>MPNKITKEALTFDDVSLIPRKSSVLPSEVSLKTQLTKNISLNIPFLSSAMDTVTESQMAIAIAKE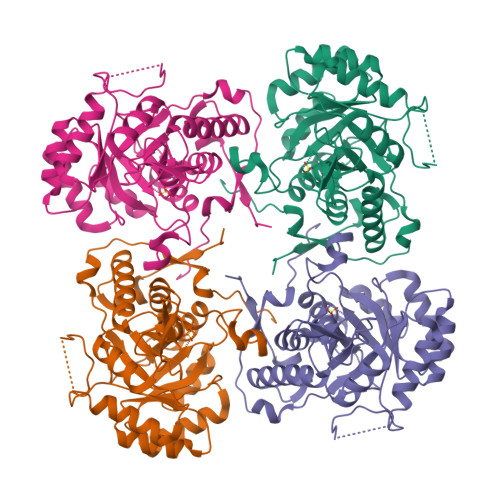GGIGIIHKNMSIEAQRKEIEKVKTYKFQKTINTNGDTNEQKPEIFTAKQHLEKSDAYKNAEHKEDFPNACKDLNNKLRVGAAVSIDIDTIERVEELVKAHVDILVIDSAHGHSTRIIELIKKIKTKYPNLDLIAGNIVTKEAALDLISVGADCLKVGIGPGSICTTRIVAGVGVPQITAICDVYEACNNTNICIIADGGIRFSGDVVKAIAAGADSVMIGNLFAGTKESPSEEIIYNGKKFKSYVGMGSISAMKRGSKSRYFQLENNEPKKLVPEGIEGMVPYSGKLKDILTQLKGGLMSGMGYLGAATISDLKINSKFVKISHSSLKESHPHDVFSIT[2x]(3S,4R,5R)-4,5-dihydroxypiperidine-3-carboxylic 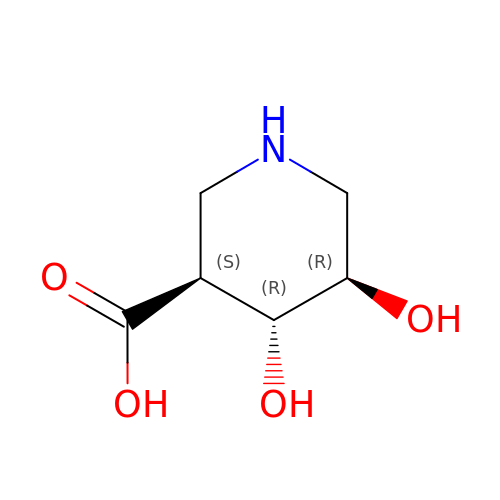acid | C6 H11 N O4 | SSMLJUWXZFXWSF-VPENINKCSA-N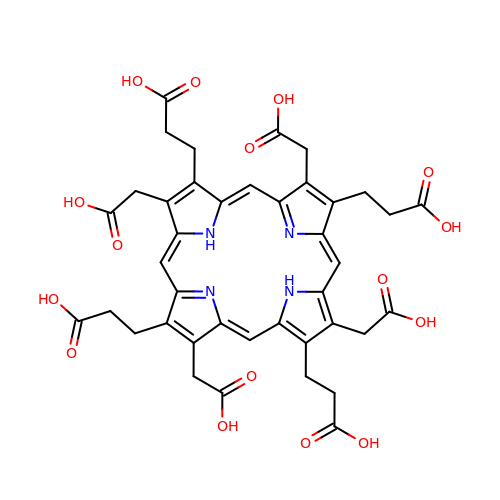3-[(1Z,9Z)-3,8,13,18-tetrakis(2-hydroxy-2-oxoethyl)-7,12,17-tris(3-hydroxy-3-oxopropyl)-21,23-dihydroporphyrin-2-yl]propanoic acid | C40 H38 N4 O16 | DAFUFNRZWDWXJP-JRHDEHKPSA-N> MDSGYSSSYAAAAGMHVVICPWLAFGHLLPCLDLAQRLASRGHRVSFVSTPRNISRLPPVRPALAPLVAFVALPLPRVEGLPDGAESTNDVPHDRPDMVELHRRAFDGLAAPFSEFLGTACADWVIVDVFHHWAAAAALEHKVPCAMMLLGSAHMIASIADRRLERAETESPAAAGQGRPAAAPTFEVARMKLIRTKGSSGMSLAERFSLTLSRSSLVVGRSCVEFEPETVPLLSTLRGKPITFLGLMPPLHEGRREDGEDATVRWLDAQPAKSVVYVALGSEVPLGVEKVHELALGLELAGTRFLWALRKPTGVSDADLLPAGFEERTRGRGVVATRWVPQMSILAHAAVGAFLTHCGWNSTIEGLMFGHPLIMLPIFGDQGPNARLIEAKNAGLQVARNDGDGS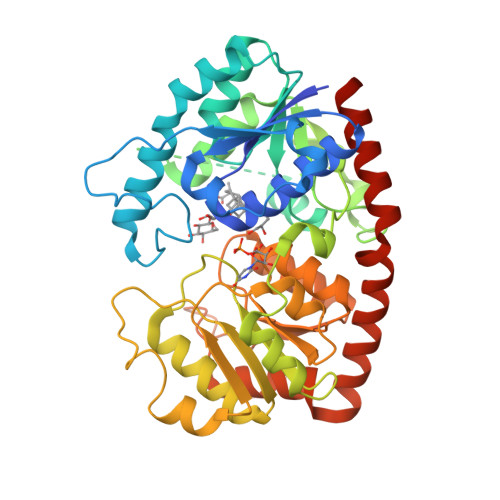FDREGVAAAIRAVAVEEESSKVFQAKAKKLQEIVADMACHERYIDGFIQQLRSYKDLEHHHHHH Porphobilinogen deaminase (PBGD; EC 2.5.1.61), also known as hydroxymethylbilane synthase (HMBS), is the third enzyme in the heme biosynthetic pathway. PBGD catalyzes four consecutive reactions to convert porphobilinogen (PBG) into hydroxymethylbilane (HMB), a linear tetrapyrrole heme precursor. The holoenzyme (Eholo) carries a dipyrromethane (DPM) cofactor, which is covalently linked to a conserved cysteine residue (Cys261 in hPBGD) through a thioether bond (Song et al., 2009). Mutations in the HMBS gene are associated with a genetic metabolic disorder known as acute intermittent porphyria (AIP), giving reduced heme production and severe metabolic and neurological symptoms (Bonkovsky et al., 2019).

In agreement with the ESI FT-ICR MS analyses of wt-hPBGD, a fully reduced covalently attached DPM occupies the active site cleft, showing a ∼120° angle between the pyrrole rings, instead of the coplanar conformation of oxidized DPM (Azim et al., 2014). The crystal structure only represents the Eholo-state and is denoted as wt-Eholo hereafter. The variability of the electron density quality as well as elevated B-factors indicate a dynamic nature of the residues Leu257–Val263 that constitute the cofactor-binding loop. Electron density is missing for the first 18 residues at the N-terminus and for the active-site loop residues Ser57–Lys74. Unfortunately, surface exposed residues in flexible sidechains, including Arg167, are not described in the electron density maps. Furthermore, both our structures contain two monomers in the asymmetric unit without indication of dimerization as also supported by the mass spectrometry results showing that except for minor dimeric forms, Eholo and the other enzyme-intermediates are monomeric. The crystallization of the wt-PBGD was performed from a mixture of intermediates, and the heterogeneity of the sample, as well as the flexible parts of the enzyme, such as the N-terminus and the loop including residues 57–74, most likely affect the quality of the data.

>GSMSGNGNAAATAEENSPKMRVIRVGTRKSQLARIQTDSVVATLKASYPGLQFEIIAMSTTGDKILDTALSKIGEKSLFTKELEHALEKNEVDLVVHSLKDLPTVLPPGFTIGAICKRENPHDAVVFHPKFVGKTLETLPEKSVVGTSSLRRAAQLQRKFPHLEFRSIRGNLNTRLRKLDEQQEFSAIILATAGLQRMGWHNRVGQILHPEECMYAVGQGALGVEVRAKDQDILDLVGVLHDPETLLRCIAERAFLRHLEGGCSVPVAVHTAMKDGQLYLTGGVWSLDGSDSIQETMQATIHVPAQHEDGPEDDPQLVGITARNIPRGPQLAAQNLGISLANLLLSKGAKNILDVARQLNDAH[2x]> GPSHEHEDKSPETVLQSAIKLEYARLVKLAQEDTPPETDYRLHHVVVYFI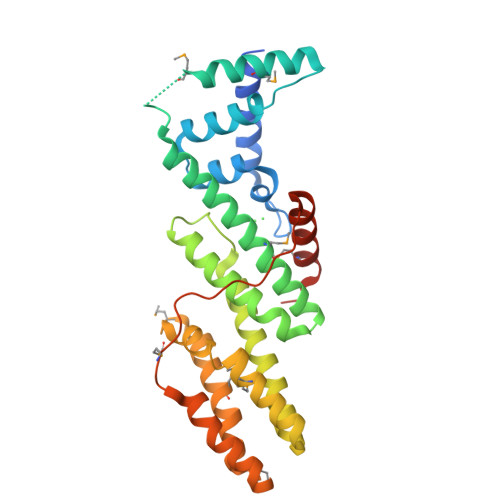QNQAPKKIIEKTLLEQFGDRNLSFDERCHNIMKVAQAKLEMIKPEEVNLEEYEEWHQDYRKFRETTMYLIIGLENFQRESYIDSLLFLICAYQNNKELLSKGLYRGHDEELISHYRRECLLKLNEQAAELFESGEDREVNNGLIIMNEFIVPFLPLLLVDEMEEKDILAVEDMRNRWCSYLGQEMEPHLQEKLTDFLPKLLDCSMEIKSFHEPPKLPSYSTHELCERFARIMLSLSRTPADGR>[5x]EWTGDNTNAYYSDEVISELHVGQIDTSPYFCIKTVKANGSGTPVVACAVSKQSIWAPSFKELLDQARYFYSTGQSVRIHVQKNIWTYPLFVNTFSANALVGLSSCSATQCFGPK;> NISDYKVMTWNLQGSSASTESKWNVNVRQLLSGTAGVDILMVQEAGAVPTSAVPTGRHIQPFGVGIPIDEYTWNLGTTSRQDIRYIYHSAIDVGARRVNLAIVSRQRADNVYVLRPTTVASRPVIGIGLGNDVFLTAHALASGGPDAAAIVRVTINFFRQPQMRHLSWFLAGDFNRSPDRLENDLMTEHLERVVAVLAPTEPTQIGGGILDYGVIVDRAPYSQRVEALRNPQLASDHYPVAFLARSCLEHHHHHH;> VDFVYRVDSTPPDVIFRDGFSLLGYNRNFQQFISGRSCSGGSSDSRYIATTSSVNQTYAIARAYYSRSTFKGNLYRYQIRADNNFYSLLPSITYLETQGGHFNAYEKTMMRLQREYVST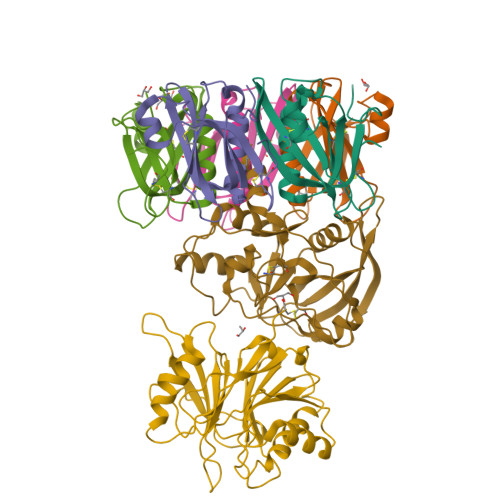LSILPENIQKAVALVYDSATGLVKDGVSTMNASYLGLSTTSNPGVIPFLPEPQTYTQQRIDAFGPLISSCFSIGSVCHSHRGQRADVYNMSFYDARPVIELILSK The genome-organizing protein p6 of Bacillus subtilis bacteriophage φ29 plays an essential role in viral development by activating the initiation of DNA replication and participating in the early-to-late transcriptional switch. These activities require the formation of a nucleoprotein complex in which the DNA adopts a right-handed superhelix wrapping around a multimeric p6 scaffold, restraining positive supercoiling and compacting the viral genome. Additionally, p6 forms dimers that bind to DNA every 24 nucleotides and interact with the viral DNA through the minor groove. In this work, we have shown that protein p6 showcases a remarkable evolutionary design that encompasses a folded core as its foundation, upon which, two structural regions play crucial roles in dimerization and oligomerization.

In a third attempt, we further truncated the initial four residues of the C-terminal tail, resulting in the p6CΔ20 variant, which readily yielded well-formed crystals, facilitating the acquisition of high quality-diffraction data. The 3D structure of p6CΔ20 was solved at 2.3 Å resolution and revealed the presence of two p6 monomers within the asymmetric unit. Both monomers assemble in an elongated tail-to-tail manner, forming a p6 dimer with maximum dimensions of 26 × 26 × 106 Å. Consequently, the main dimerization interface (DI) results from the precise packing of the α2 helices from both protomers. Dimerization occurs via an extensive hydrophobic interface, covering ∼1000 Å2 of accessible surface area (ASA) including 15% of the total ASA of each subunit. Superimposition of the two chains of the p6CΔ20 dimer (by aligning the main folded core) revealed notable differences primarily concentrated in two regions. The first one (R1, corresponding to region ii on Figure 2A) shows a significant displacement of the β-hairpin in Monomer 1 compared to Monomer 2 (with a tilt of ∼29°), indicating substantial structural plasticity in this region, crucial for p6 oligomerization as discussed in the next section. In Monomer 2, this region is kinked and displaced ∼47° compared to Monomer 1 and constitutes another source of significant structural plasticity that defines a ‘hinge region’ [predicted by the server HINGEprot (83)], involving residues E7 and E67 from β1 and β4; respectively. Interestingly, crystal packing analysis of p6CΔ20 structure unveiled that the protein crystallized as an oligomer. In this oligomer, the p6CΔ20 dimers are the building blocks that create a chain of linked dimers in a head-to-head fashion. This arrangement results in a superhelix with six p6CΔ20 molecules per turn, measuring ∼60 Å in diameter and 230 Å in height.

>[2x]AKMMQREITKTTVNVAKMVMVDGEVQVEQLPSETFVGNLTMEQAQWRMKRKYKGEPVQVVSVEPNTEVYELPVEKFLEVATVR>[4x]SQPAFPVQILPYLYLGCAKDS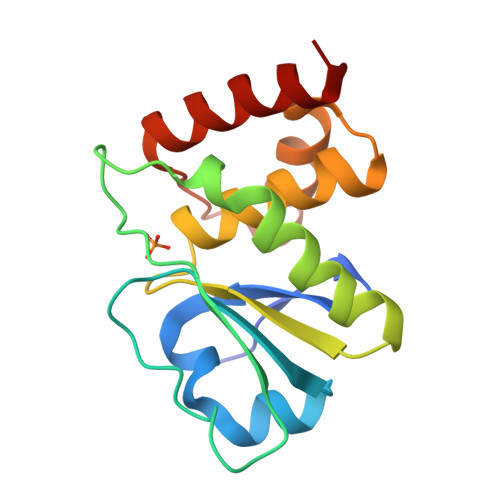TNLDVLGKYGIKYILNVTPNLPNAFEHGGEFTYKQIPISDHWSQNLSQFFPEAISFIDEARSKKCGVLVHSLAGISRSVTVTVAYLMQKMNLSLNDAYDFVKRKKSNISPNFNFMGQLLDFERTLGLS> DEIIDETDNLYVSQGPGVDISGDVNLTDFDKIGWPNVEAVQSYQREFNAVSNIFDTIYPIGTIYENAVNPNNPVTYMGFGSWKLFGQGKVLVGWNEDISDPNFALNNNDLDSGGNPSHTAGGTGGSTSVTLENTNLPATE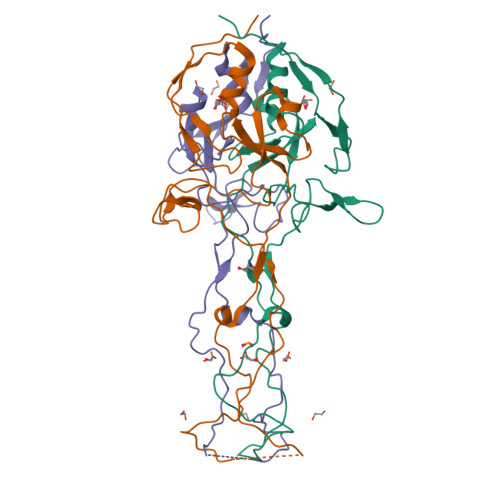TDEEVLIVDENGSVIVGGCQYDPDESGPIYTKYREAKASTNSTHTPPTSITNIQPYITVYRWIRIA>ALAGTIIAGASLTFQVLDKVLEELGKVSRKIAVGIDNESGGTWTALNAY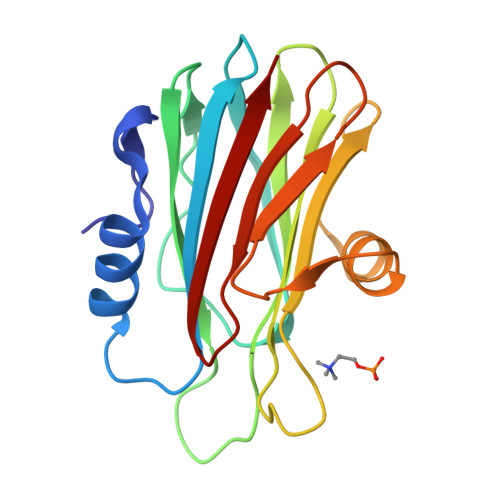FRSGTTDVILPEFVPNTKALLYSGRKDTGPVATGAVAAFAYYMSSGNTLGVMFSVPFDYNWYSNWWDVKIYSGKRRADQGMYEDLYYGNPYRGDNGWHEKNLGYGLRMKGIMTSAGEAKMQIKISR[2x]The TGF-β ligands are dimers and initiate signal transduction by forming a signalling complex with two copies of a type I receptor and two copies of a type II receptor; all are single-pass transmembrane proteins containing a small extracellular ligand-binding domain (ECD) and an intracellular kinase domain (ICD). Upon signalling complex formation, the constitutively active type II receptor phosphorylates and activates the type I receptor; subsequently the type I receptor phosphorylates Smad1/5 or Smad2/3 to regulate transcriptional responses. For example, ActRIIA/B bind to and mediate the signalling from both activin ligands and some BMP ligands, whereas BMPRII is the low-affinity type II receptor for over 15 BMP ligands. Of note, BMPRII is particularly highly expressed in lung vascular endothelial cells, where it mediates the signalling from circulating BMP9 and BMP10.

In addition, we solved the crystal structure of the ALK1:BMP10:BMPRII ternary signalling complex. There are 4 copies each of BMP10, ALK1 and BMPRII monomers in an asymmetric unit, assembled into two copies of BMP10 ternary signalling complexes. Complex 1 (cpx1) contains chains A, B, E, F, I and J, and cpx2 contains chains C, D, G, H, K and L. In the ternary complex, while good densities were observed for all BMP10 and ALK1 chains, densities for BMPRII were relatively weaker. Overall, the BMPRII-signalling complex assembly resembles the reported BMP family complexes, in which ALK1 binds BMP10 at the wrist epitope and BMPRII binds at the knuckle epitope. No direct contact is present between ALK1 and BMPRII. Overlaying the ALK1:BMP10 portion of the ternary complexes onto the previously reported ALK1:BMP10 complex showed no significant conformational change. The buried surface areas at the interfaces from the ternary complexes are generally smaller than those from the binary complexes with only one exception, but in the same range as the BMP9:ActRIIB interface in the ternary signalling complexes. We questioned whether fewer interface interactions and a smaller interface area would translate to weaker BMP10:BMPRII interactions in the ternary complexes. In the surface plasmon resonance (SPR) binding assay, indeed, BMP10 bound to BMPRII-Fc surface with ~5 fold weaker affinity when ALK1 was present. The fact that the extended conformation of BMP10 is only observed in the ternary not the BMP10:BMPRII binary complex suggests that BMP10 type II surface in the ternary complex may not be the optimum surface for BMPRII binding.

>[4x]NAKGNYCKRTPLYIDFKEIGWDSWIIAPPGYEAYECRGVCNYPLAEHLTPTKHAIIQALVHLKNSQKASKACCVPTKLEPISILYLDKGVVTYKFKYEGMAVSECGCR;>DPVKPSRGPLVTCTCESPHCKGPTCRGAWCTVVLVREEGRHPQEHRGCGNLHRELCRGRPTEFVNHYCCDSHLCNHNVSLVLEATQPPSEQPGTDGQ[4x];>SQNQERLCAFKDPYQQDLGIGESRISHENGTILCSKGSTCYGLWEKSKGDINLVKQGCWSHIGDPQECHYEECVVTTTPPSIQNGTYRFCCCSTDLCNVNFTENFPPPDTTPLSPPHSFNRDET[4x]> GPLGSPGRPMPINRPNLNLNIPPLNIVAAYDGAEIPSTNKHLKNNFNSLHNQMRKMPVSHFKEALDVPDYSGMRQSGFFAMSQGFQLNNHGYDVFIHARRESPQSQGKFAGDKFHISVLRDMVPQAFQALSGLLFSEDSPVDKWKVTDMEKVVQQARVSLGAQFTLYIKPDQENSQYSASFLHKTRQFIECLESRLSENGVISGQCPESDVHPENWKYLSYRNELRSGRDGGEMQRQALREEPFYRLMT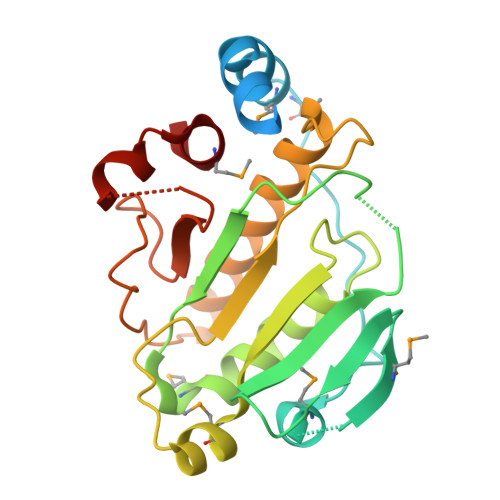E>MCLEDSDAGASNEYDSSPAAWNKEDFPWSGKVKDILQNVFKLEKFRPLQLETINVTMAGKEVFLVMPTGGGKSLCYQLPALCSDGFTLVICPLISLMEDQLMVLKQLGISATMLNASSSKEHVKWVHAEMVNKNSELKLIYVTPEKIAKSKMFMSRLEKAYEARRFTRIAVDEVHCCSQWGHDFRPDYKALGILKRQFPNASLIGLTATATNHVLTDAQKILCIEKCFTFTASFNRPNLYYEVRQKPSNTEDFIEDIVKLINGRYKGQSGIIYCFSQKDSEQVTVSLQNLGIHAGAYHANLEPEDKTTVHRKWSANEIQVVVATVAFGMGIDKPDVRFVIHHSMSKSMENYYQESGRAGRDDMKADCILYYGFGDIFRISSMVVMENVGQQKLYEMVSYCQNISKCRRVLMAQHFDEVWNSEACNKMCDNCCKDSAFERKNITEYCRDLIKILKQAEELNEKLTPLKLIDSWMGKGAAKLRVAGVVAPTLPREDLEKIIAHFLIQQYLKEDYSFTAYATISYLKIGPKANLLNN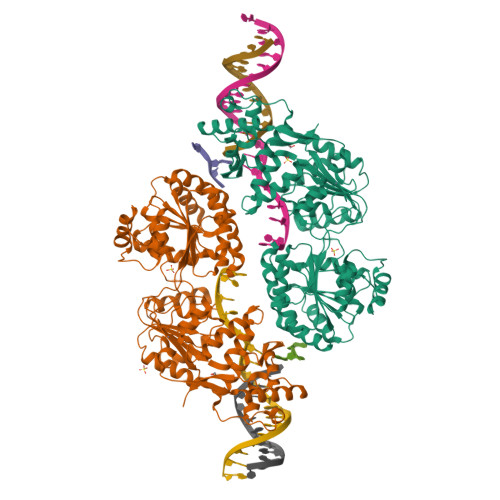EAHAITMQVTKSTQNSFRAESSQTCHSEQGDKKMEAENLYFQSHHHHHHDYKDDDDK[2x]> YFAYDRRXLSNNXRNY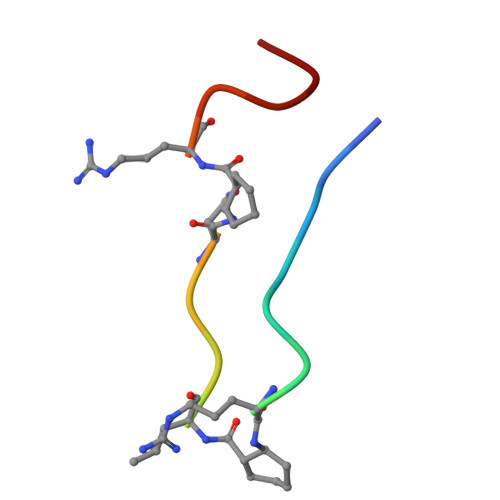CG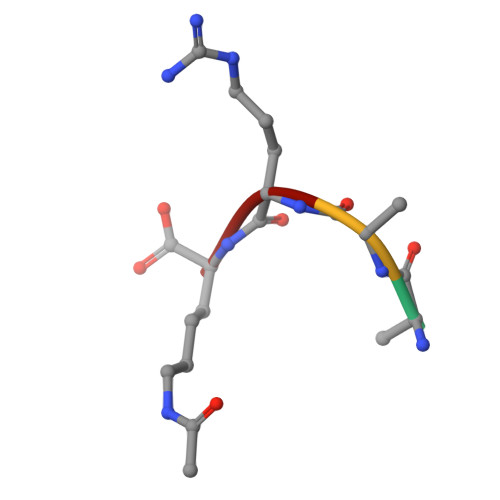> AARK Despite the abundance of PARP1, most of the PAR generated by DNA damage is rapidly degraded, with a half-life of less than 1 min by poly (ADP-ribose) glycohydrolase (PARG). The radio-resistant bacterium D. radiodurans encodes a PARG homolog, DrPARG, whose expression is upregulated after radiation damage, so it might play an important role in DNA repair. Our study demonstrates that DrPARG is involved in catalyzing the breakdown of endogenous PAR and DNA repair in D. radiodurans. From observing the structural peculiarities of DrPARG, we show that although previously thought to be an obligate exo-glycohydrolase, bacterial PARG could exert both exo- and endo-glycohydrolase functions.

Therefore, we attempted to obtain crystals of DrPARG in complex with ADP-ribose. Crystals were found in several similar conditions, but they belonged to different space groups. The monoclinic crystals of DrPARG in the ADP-ribose bound form gave the highest-resolution X-ray diffraction with space group P21 refined to 1.97 Å resolution. The missing 11 residues (100GGGFLGGAQAQ110) from the catalytic loop of the apo-form structure could be defined as a loop region in the ADP-ribose-bound form. As compared with the apo-form structure, the bound form structure of DrPARG showed additional secondary structures: a short β-strand (denoted β4′) following β4, extension of β5, and an α-helix (denoted α4′) preceding α4. Like previously reported PARGs, coordination of ADP-ribose involves serial hydrogen bond formations and hydrophobic interactions provided by surrounding amino acid residues in DrPARG. The side chain of Asp113 located in the α4 helix contacts the N6 atom of the pyrimidine ring in the adenine moiety via direct hydrogen bonding. Oxygen atoms of the pyrophosphate in ADP-ribose contact surrounding residues via hydrogen bonding with nitrogen atoms in the main chain of Gln110, Gly224, Gly226, Val227, and Phe228. In terms of generally similar binding mode of ADP-ribose among DrPARG, TcPARG, and PARG structures in complex with ADP-ribose from Homo sapiens (HsPARG), the conserved catalytical residue Glu112 of DrPARG does not form a hydrogen bond with 1′-OH of the ribose″ moiety via its side chain. However, like in HsPARG, we observed a solvent-accessible 2′-OH of the ribose′ moiety in DrPARG, which suggests the internal binding of PAR polymers to DrPARG.

>[2x]VRLPGLAAMRQGTRLFTPEQGEDLREALRRRRGSFQTTCEVTSETTFAAARRLREKASALAALNFASAKNPGGGFLGGAQAQEEDLCRGSGLYFSLTSPQAEPYYAVNRQSHSALYTDHLIYSPQVPIFRDDAGQLLPAPVPVNIITAPAPNAGAVAQSRPEQLPQVLPTLRERARRVLGVAAWMEQTHLVLGAWGCGVFRNDPAGVARTFRELLEGEAQGAFEHVTFAVLDNHPQHPTLGAFRRELESLCLP>[2x]EQARPADDALAALGAQLFVDPALSRNATQSCATCHDPARAFTDPREGKAGLAVSVGDDGQSHGDRNTPTLGYAALVPAFHRDANGKYKGGQFWDGRADDLKQQAGQPMLNPVQMAMPDRAAVAARLRDDPAYRTGFEALFGKGVLDDPERAFDAAAEALAAYQATGEFSPFDSKYDRVMRGEEKFTPLEEFGYTVFITWNCRLCHMQRKQGVAERETFTNFEYHNIGLPVNETAREASGLGADHVDHGLLARPGIEDPAQSGRFKVPSLRNVAVTGPYMHNGVFTDLRTAILFYNKYTSRRPEAKINPETGAPWGEPEVARNLSLAELQSGLMLDDGRVDALVAFLETLTDRRYEPLLEESRAAQKDHHHHHH;>[2x]ADAPAGTDPRAKWVPQDNDIQACDYWRHCSIDGNICDCSGGSLTNCPPGTKLATASWVASCYNPTDGQSYLIAYRDCCGYNVSGRCPCLNTEGELPVYRPEFANDIIW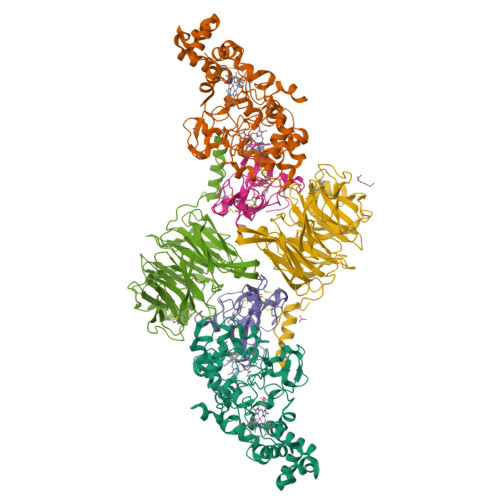CFGAEDDAMTYHCTISPIVGKASHHHHHH;>[2x]DAPEAETQAQETQGQAAARAAAADLAAGQDDEPRILEAPAPDARRVYVNDPAHFAAVTQQFVIDGEAGRVIGMIDGGFLPNPVVADDGSFIAHASTVFSRIARGERTDYVEVFDPVTLLPTADIELPDAPRFLVGTYPWMTSLTPDGKTLLFYQFSPAPAVGVVDLEGKAFKRMLDVPDCYHIFPTAPDTFFMHCRDGSLAKVAFGTEGTPEITHTEVFHPEDEFLINHPAYSQKAGRLVWPTYTGKIHQIDLSSGDAKFLPAVEALTEAERADGWRPGGWQQVAYHRALDRIYLLVDQRDEWRHKTASRFVVVLDAKTGERLAKFEMGHEIDSINVSQDEKPLLYALSTGDKTLYIHDAESGEELRSVNQLGHGPQVITTADMG>MIDLKQYEFWFLVGSQYLYGLETLKKVEQQASKIVDSLNDDPIFPSKIVLKPVLKSSSEITEIFEKANADPKCAGVIVWMHTFSPSKMWIRGLSINKKPLLHLHTQYNREIPWDTIDMDYMNLNQSAHGDREHGFIHARMRLPRKVVVGHWEEKEVREKIAKWMRVACAIQDGRMGQIVRFGDNMREVASTEGDKVEAQIKLGWSINTWGVGELAERVKAVPEREVEELLKEYREKYIMPEDEYSLKAIREQAKIEIALREFLKEKNAVGFTTTFEDLHDLPQLPGLAVQRLME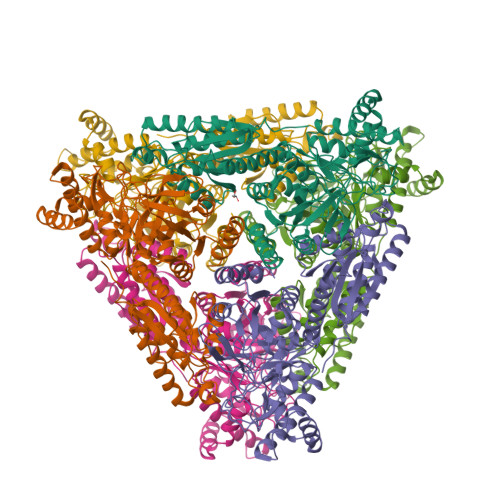EGYGFGAEGDWKAAGLVRAIKVMGTSLPGGTSFMEDYTYHLTPGNELVLGAHMLEVCPTIAKEKPRIEVHPLSIGGKADPARLVFDGQEGPAVNASIVDMGNRFRLVVNKVLSVPIERKMPKLPTARVLWKPLPDFKRATTAWILAGGSHHTAFSTAIDVEYLIDWAEALEIEYVVIDENLDLEDFKKELRWNELYWGLLKR[12x]> MQDAITAVINSSDVQG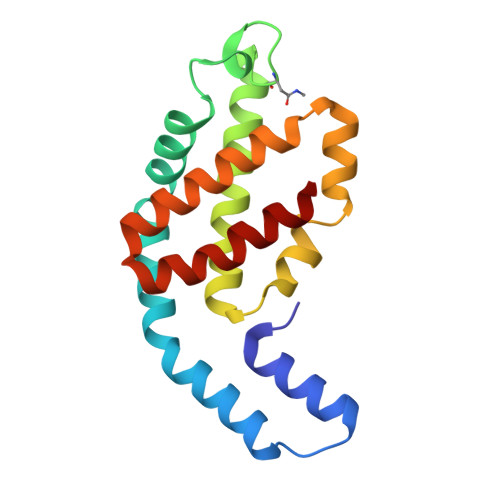KYLDGSAMEKLKAYFQTGELRVRAATTISANAAEIVKDAVAKSLLYSDITRPGGNMYTTRRYAACIRDLDYYLRYSTYAMLAGDPSILDERVLNGLKETYNSLGVPVGATVQAIQAMKEVTATLVGADAGKEMGVYFDYICSGLS>GMNIISQNTAFGGMQGVFSHQSETLKSEMTFAVYVPPKAIHEPCPVVWYLSGLTCTHANVMEKGEYRRMASELGLVVVCPDTSPRGNDVPDELTNWQMGKG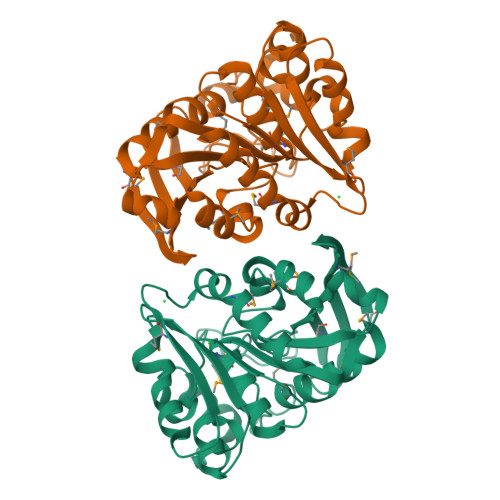AGFYLDATEEPWSEHYQMYSYVTEELPALIGQHFRADMSRQSIFGHSMGGHGAMTIALKNPERFKSCSAFAPIVAPSSADWSEPALEKYLGADRAAWRRYDACSLVEDGARFPEFLIDQGKADSFLEKGLRPWLFEEAIKGTDIGLTLRMHDRYDHSYYFISTFMDDHLKWHAERLG[6x]>[2x]MEPRMESCLAQVLQKDVGKRLQVGQELIDYFSDKQKSADLEHDQTMLDKLVDGLATSWVNSSNYKVVLLGMDILSALVTRLQDRFKAQIGTVLPSLIDRLGDAKDSVREQDQTLLLKIMDQAANPQYVWDRMLGGFKHKNFRTREGICLCLIATLNASGAQTLTLSKIVPHICNLLGDPNSQVRDAAINSLVEIYRHVGERVRADLSKKGLPQSRLNVIFTKFDEVQKSGNMIQSANDKNFDDEDSVDGNRPSSASS

Two prime animal MAP families that bind tubulin and are recruited to microtubule plus ends by EB proteins (either directly or indirectly) are the Cytoplasmic Linker-Associated Protein (CLASP) family and the XMAP215 family of microtubule polymerases. While XMAP215 family members promote microtubule polymerization, CLASP family members promote microtubule pause, potentiate rescue, and limit catastrophe. While the CLASP and XMAP215 families differentially affect microtubule dynamics, they both employ an array of tubulin-binding TOG domains to regulate the microtubule polymer. While mammalian XMAP215 family members contain an N-terminal pentameric TOG domain array, mammalian CLASPs contains three TOG domains (TOG1-3) followed by a C-terminal CLIP-170 interaction domain (CLIP-ID).

To determine the structure of H.s. CLASP1 TOG1 we crystallized a selenomethionine-substituted construct embodying residues 1 to 257 and collected a 2.15 Å resolution single wavelength anomalous diffraction dataset. Crystals belong to the space group P21 and contain two protomers in the asymmetric unit. The structure was refined to R and Rfree values of 19.0% and 24.4% respectively. CLASP TOG1 is an α-solenoid structure approximately 65 Å in length, consisting of six HRs designated HR A through F. The second HR triad (HRs D-F) is translated relative to the axis of the first HR triad, introducing a jog in the α-solenoid that gives the domain a flat, paddle-like architecture, rather than an elongated spiral common to other α-solenoid structures. Interestingly, while XMAP215 family TOG domains are primarily conserved across the HR A-C intra-HEAT loops, animal CLASP family TOG1 conservation is primarily focused along the surface formed by the HR C-E intra-HR loops. CLASP1 TOG1 superimposes on the Stu2 TOG2-αβ-tubulin structure surprisingly well, with its intra-HEAT loops positioned to complement the surface of the tubulin heterodimer. CLASP1 TOG1 has distinct determinants across the intra-HR loops that likely explain why no tubulin or microtubule-binding activity has been detected for animal CLASP family TOG1 domains. Instead of binding tubulin, the animal CLASP family TOG1 domain’s conserved intra-HR loops may be involved in binding a kinetochore factor, relieving the auto-inhibition of the CLASP family TOG2 domain’s activity, binding actin, or a yet to be determined factor.>[2x]MGSMCPKDWKLFGSHCYLVPTVFSSASWNKSEENCSRMGAHLVVIHSQEEQDFITGILDIHAAYFIGLWDTGHRQWQWVDQTPYEESVTFWHNGEP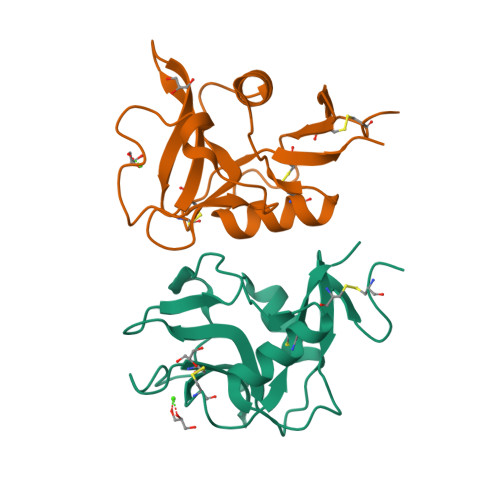SSDNEKCVTVYYRRNIGWGWNDISCNLKQKSVCQMKKINL9-chloro-7-(2,6-difluorophenyl)-N-{4-[(4-methylpiperazin-1-yl)carbonyl]phenyl}-5H-pyrimido[5,4-d][2]benzazepin-2-amine 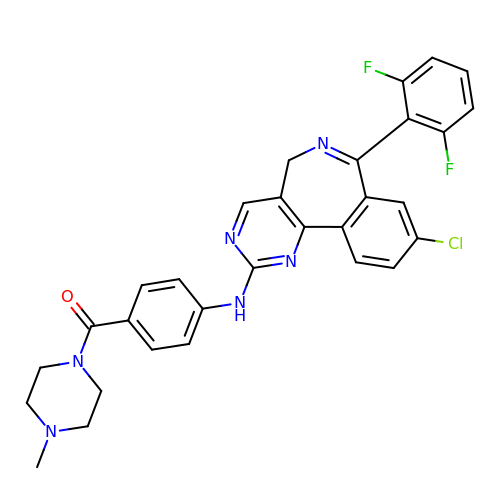| C30 H25 Cl F2 N6 O | SEYRFEUDBMZPCH-UHFFFAOYSA-N>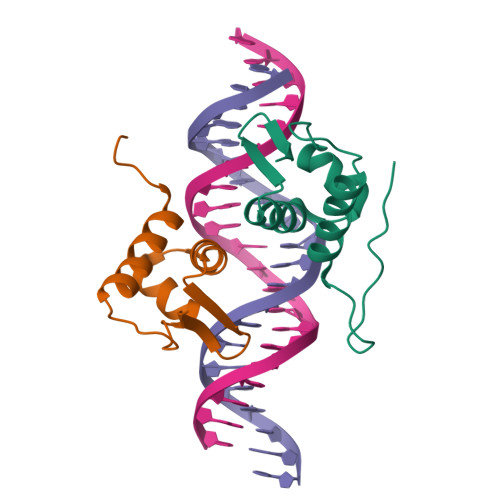[2x]MHHHHHHLEVLFQGPLGSEFMLPKYAQVKEEISSWINQGKILPDQKIPTENELMQQFGVSRHTIRKAIGDLVSQGLLYSVQGGGTFVA>GMRNPSEDHMMRTPYQIVADHYAASDRHDPAAMMADIAPAIEWTEMAGFPCAGTYRSADEIVRNVFRRLGEEWDGYTF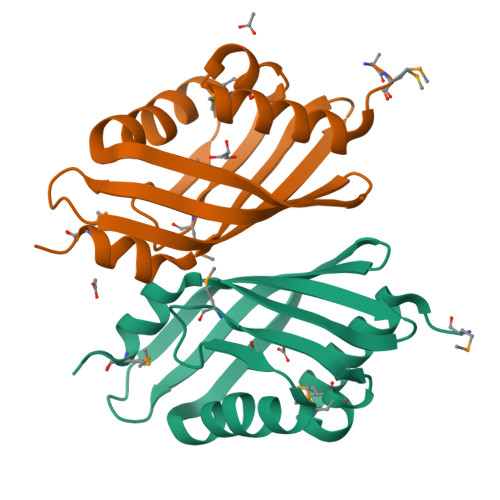KLDALHDAGDTVIGVGRYSGTYRRTGKSFECRVAHVWRVDAGKIVHFEQFTDTLLVAQAMQP[2x]> GSGI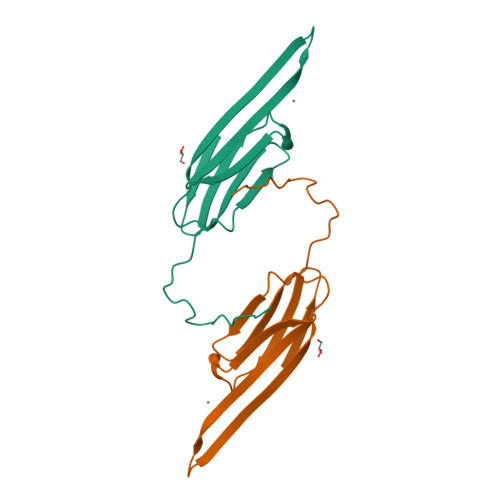SEVRSDRDKFVIFLDVKHFSPEDLTVKVQEDFVEIHGKHNERQDDHGYISREFHRRYRLPSNVDQSALSCSLSADGMLTFSGPKIPSGVDAGHSERAIPVSR METHYLENE ADP-BETA-XYLOSE | C16 H25 N5 O13 P2 | 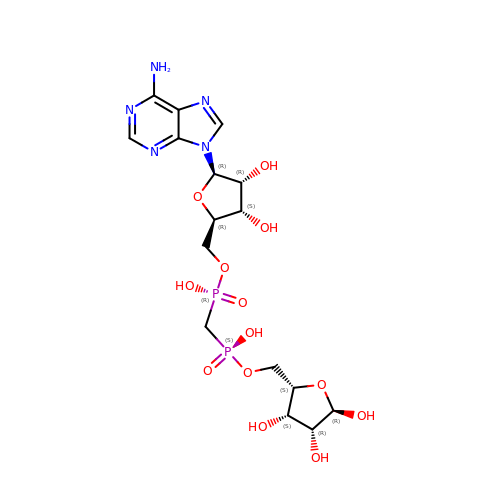ZPZRETFSCSWNDT-CAUCCWOKSA-N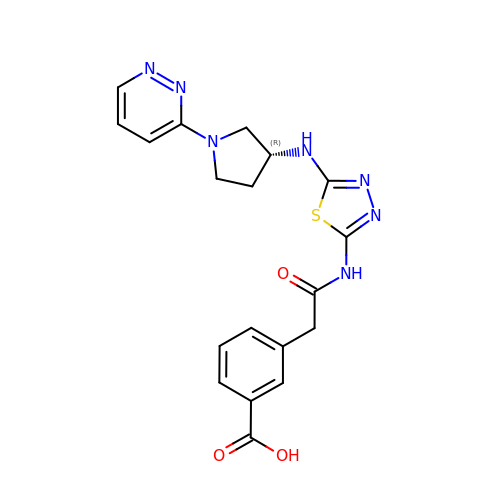3-[2-oxidanylidene-2-[[5-[[(3R)-1-pyridazin-3-ylpyrrolidin-3-yl]amino]-1,3,4-thiadiazol-2-yl]amino]ethyl]benzoic acid | C19 H19 N7 O3 S | HMCXTWYQJBJKRJ-CQSZACIVSA-N> TGYISIDAMKKFLGELHDFIPGTSGYLAYHVQNE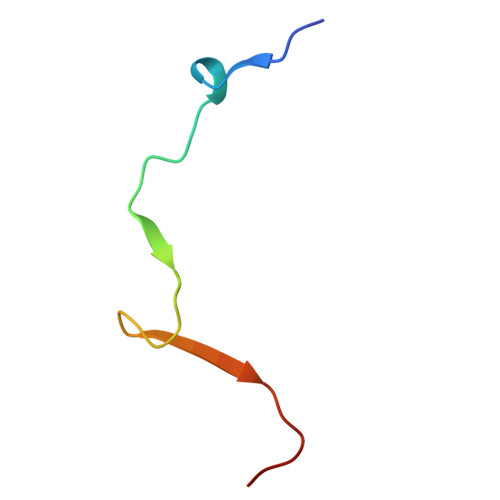IN2-(6-methylpyridin-2-yl)-N-pyridin-4-ylquinazolin-4-amine 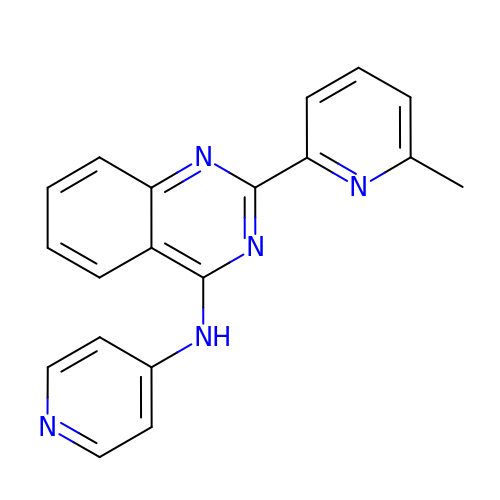| C19 H15 N5 | JONFDFIXMPXTRH-UHFFFAOYSA-N> MAHHHHHHVSDIPSDLHYTA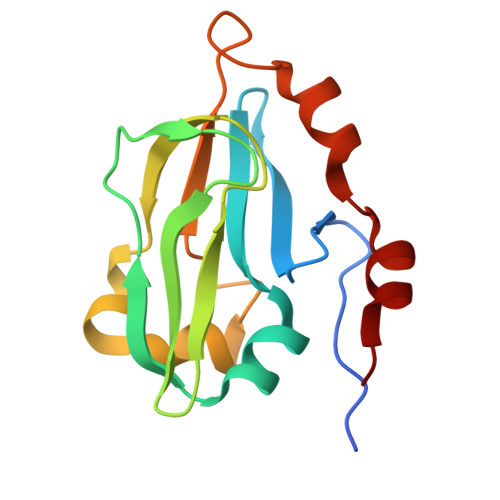EHEWIRRSGDDTVRVGITDYAQSALGDVVFVQLPVIGTAVTAGETFGEVESTKSVSDLYAPISGKVSEVNSDLDGTPQLVNSDPYGAGWLLDIQVDSSDVAALESALTTLLDAEAYRGTLTE>[2x]MDQFVGLHMIYTYENGWEYEIYI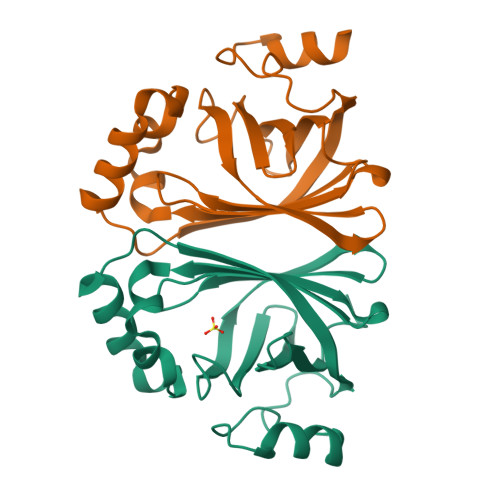KNDHTIDYRIHSGMVGGRWVRDQEVNIVKLTKGVYKVSWTEPTGTDVSLNFMPEEKRMHGVIFFPKWVHERPDITVCYQNDYIDLMKESREKYETYPKYVVPEFADITYIHHAGVNDETIIAEAPYEGMTDEIRAGRK4-methyl-5-(1-methyl-1H-imidazol-2-yl)-1,3-thiazol-2-amine 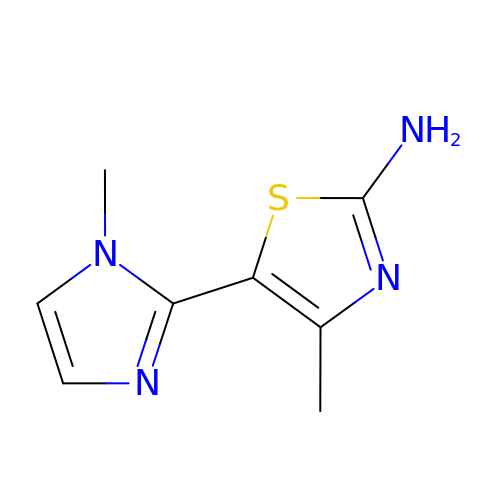| C8 H10 N4 S | MHYCRLDCEBMUQM-UHFFFAOYSA-N For this analysis we used Cowpea Mosaic Virus (CPMV), a plant virus from the order Picornavirales that has been used extensively in biotechnology and as a model for single-stranded RNA viruses more generally. Affimer proteins are novel affinity reagents which mimic the molecular recognition of antibodies, but can be isolated quickly and produced recombinantly. Affimer proteins are small (11 kDa, 3 nm in diameter), stable (70 °C < Tm < over 100 °C), monomeric proteins that lack disulphide bonds. Their structure consists of a single α-helix and four β-strands, with the molecular recognition sites being located within two variable loops, each up to nine amino acids in length. We have analysed the structure of CPMV in complex with the Affimer reagent using cryoEM revealing the binding site of the Affimer at the 2-fold symmetry axis of the viral capsid to the L subunit.

Anti-CPMV Affimer 3 was selected as it did not cause appreciable aggregation or clumping of CPMV particles in negative stain screens. To overcome this issue CPMV was applied to lacey carbon grids overlaid with a thin (<3 nm) layer of carbon. This causes the CPMV particles to be immobilized on the carbon support, anti-CPMV Affimer 3 was subsequently applied, excess solution was removed and the grid was finally washed prior to blotting and plunge freezing (see Methods and18 for more details). The global resolution of the resulting structure was 3.4 Å. The viral capsid has the highest resolution, and previous atomic models for the L and S subunit fit into the density with clear resolution of the bulky side-chains in both capsid proteins. The L subunits (green) interact at the 2-fold symmetry axis of the icosahedral capsid and here we can see additional density that is attributed to anti-CPMV Affimer 3 (purple). Due to the icosahedral averaging applied during image processing and structure determination, these locations have two-fold symmetry applied, which is appropriate for the viral CP, but not for the bound Affimer. As a result, the non-two-fold symmetric Affimer structure is inappropriately averaged meaning there is not clear density for the backbone of the Affimer and we are unable to map the position of individual amino acids. EM density is visualized for the alpha helical domain of the Affimer with the base of the helix bound at the interface between two L subunits. Previous structural analysis of Affimer proteins has shown the location of the variable loop. Due to the location of the variable loops, we propose that the N-terminus of the Affimer reagent is facing down into the capsid as this would allow the Affimer variable loops to bind to a portion of the L subunit in the CPMV capsid.

>[4x]GPVCAEASDVYSPCMIASTPPAPFSDVTAVTFDLINGKITPVGDDNWNTHIYNPPIMNVLRTAAWKSGTIHVQLNVRGAGVKRADWDGQVFVYLRQSMNPESYDARTFVISQPGSAMLNFSFDIIGPNSGFEFAESPWANQTTWYLECVATNPRQIQQFEVNMRFDPNFRVAGNILMPPFPLSTETPPL;>[4x]MEQNLFALSLDDTSSVRGSLLDTKFAQTRVLLSKAMAGGDVLLDEYLYDVVNGQDFRATVAFLRTHVITGKIKVTATTNISDNSGCCLMLAINSGVRGKYSTDVYTICSQDSMTWNPGCKKNFSFTFNPNPCGDSWSAEMISRSRVRMTVICVSGWTLSPTTDVIAKLDWSIVNEKCEPTIYHLADCQNWLPLNRWMGKLTFPQGVTSEVRRMPLSIGGGAGATQAFLANMPNSWISMWRYFRGELHFEVTKMSSPYIKATVTFLIAFGNLSDAFGFYESFPHRIVQFAEVEEKCTLVFSQQEFVTAWSTQVNPRTTLEADGCPYLYAIIHDSTTGTISGDFNLGVKLVGIKDFCGIGSNPGIDGSRLL;> ENSLEIEELARFAVDEHNKKENALLEFVRVVKAKEQVVAGTMYYLTLEAKDGGKKKLYEAKVWVKPWENFKELQEFKPV> LQDPCSNCPAGTFCDNNRNQICSPCPPNSFSSAGGQRTCDICRQCKGVFRTRKECSSTSNAECDCTPGFHCLGAGCSMCEQD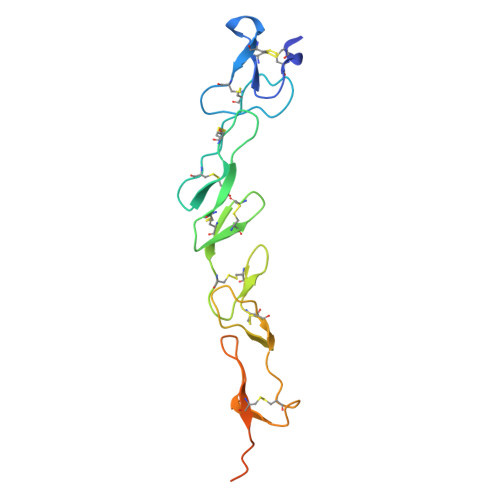CKQGQELTKKGCKDCCFGTFNDQKRGICRPWTNCSLDGKSVLVNGTKERDVVCGPSPADLSPGASSVTPPAPAREHHHHHH>MAEKNYVMAIDQGTTSSRAIIFDRNGKKIGSSQKEFPQYFPKSGWVEHNANEIWNSVQSVIAGAFIESGIRPEAIAGIGITNQRETTVVWDKTTGQPIANAIVWQSRQSSPIADQLKVDGHTEMIHEKTGLVIDAYFSATKVRWLLDNIEGAQEKADNGELLFGTIDSWLVWKLTDGQVHVTDYSNASRTMLYNIHKLEWDQEILDLLNIPSSMLPEVKSNSEVYGHTRSYRFYGSEVPIAGMAGDQQAALFGQMAFEKGMIKNTYGTGAFIVMNTGEEPQLSDNDLLTTIGYGINGKVYYALEGSIFVAGSAIQWLRDGLRMIETSPQSEELAAKAKG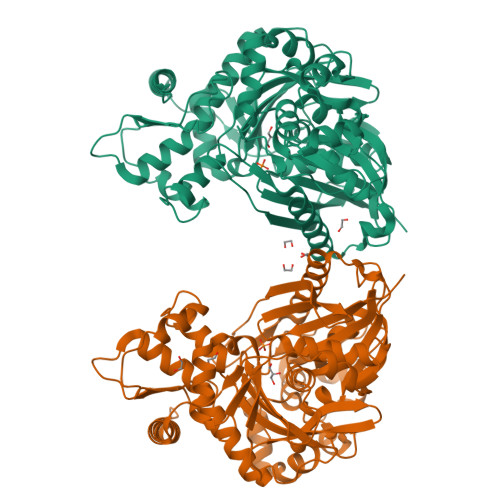DNEVYVVPAFTGLGAPYWDSEARGAVFGLTRGTTKEDFVRATLQAVAYQSKDVIDTMKKDSGIDIPLLKVDGGAAKNDLLMQFQADILDIDVQRAANLETTALGAAYLAGLAVGFWKDLDELKSMAEEGQMFTPEMPAEERDNLYEGWKQAVAATQTFKFKAKKEGE[2x]> NRWQFKNMISCTVPSRSWWDFA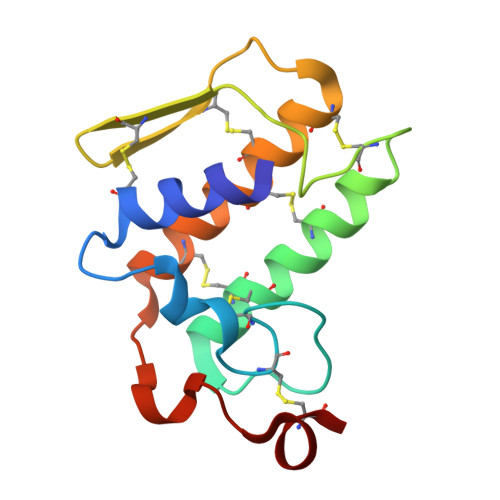DYGCYCGRGGSGTPVDDLDRCCQVHDNCYNEAEKISGCNPRFRTYSYECTAGTLTCTGRNNACAASVCDCDRLAAICFAGAPYNDNNYNIDLQARCN> ISEFDYKDHDIDYKDDDDKWIMSLSIKELYYTKDKSINNVNLADGNYVVNRGDGWILSRQNQNLGGNISNNGCTAIVGDLRIRETATPYYYPTASFNEEYIKNNVQNVFANFTEASEIPIGFEFSKTAPSNKSLYMYLQYTYIRYEIIKVLQNTVTERAVLYVPSLGYVKSIEFNSEEQIDKNFYFTSQDKCIL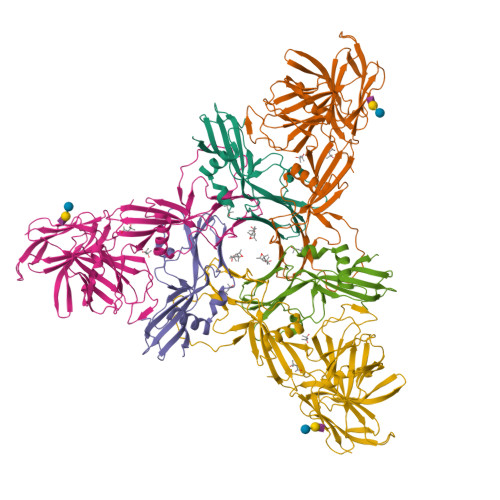NEKFIYKKIDDTITVKESKNSNNNINFNTS;> QTILPYPNGLYVINKGDGYMRTNDKDLIGTLLIESSTSGSIIQPRLRNTTRPLFNTSNPTIFSQEYTEARLNDAFNIQLFNTSTTLFKFVEEAPTNKNISMKVYNTYEKYELINYQNGNIDDKAEYYLPSLGKCEVSDAPSPQAPVVETPVDQDGFIQTGPNENIIVGVINPSENIEEISTPIPDDYTYNIPTSIQNNACYVLFKVNTTGVYKITTKNNLPPLIIYEAIGSSNRNMNSNNLSNDNIKAIKYITGLNRSDAKSYLIVSLFKDKNYYIRIPQISSSTTSQLIFKRELGNISDLADSTVNILDNLNTSGTHYYTRQSPDVGNYISYQLTIPGDFNNIASSIFSFRTRNNQGIGTLYRLTESINGYNLITINNYSDLLNNVEPISLLNGATYIFRVKVTELNNYNIIFDAYRNS>[2x]MRILVTNDDGIQSKGIIVLAELLSEEHEVFVVAPDKERSATGHSITIHVPLWMKKVFISERVVAYSTTGTPADCVKLAY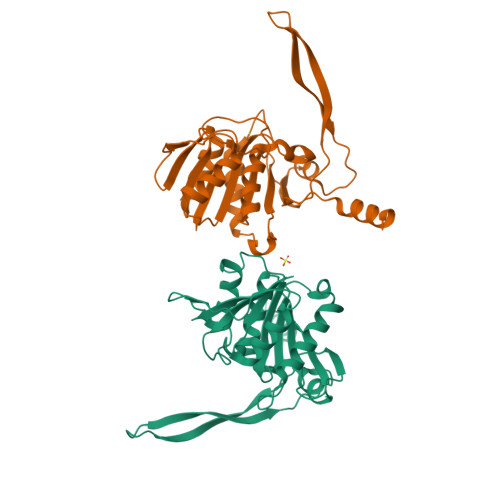NVVMDKRVDLIVSGVNRGPNMGMDILHSGTVSGAMEGAMMNIPSIAISSANYESPDFEGAARFLIDFLKEFDFSLLDPFTMLNINVPAGEIKGWRFTRQSRRRWNDYFEERVSPFGEKYYWMMGEVIEDDDRDDVDYKAVREGYVSITPIHPFLTNEQCLKKLREVYD> ETITVSTPIKQIFPDDAFAETIKANLKKKSVTDAVTQNELNSIDQIIANNSDIKSVQGIQYLPNVRYLALGGNKLHDISALKELTNLTYLILTGNQLQSLPNGVFDKLTNLKELVLVENQLQSLPDGVFDKLTNLTYLYLYHNQLQSLPKGVFDKLTNLT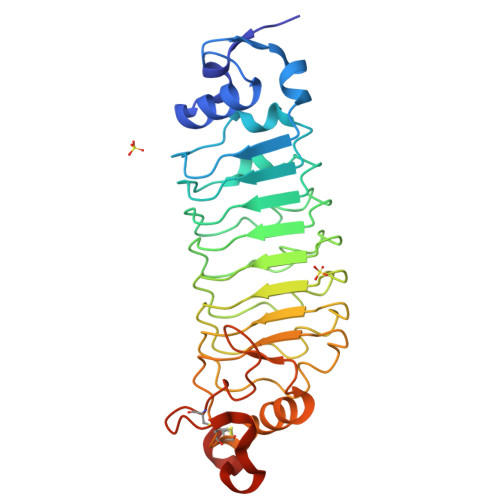RLDLDNNQLQSLPEGVFDKLTQLKQLSLNDNQLKSVPDGVFDRLTSLTHIWLLNNPWDCACSDILYLSRWISQHPGLVFGYLNLDPDSARCSGTNTPVRAVTEASTSPSKCPGHHHHHH> MSLFK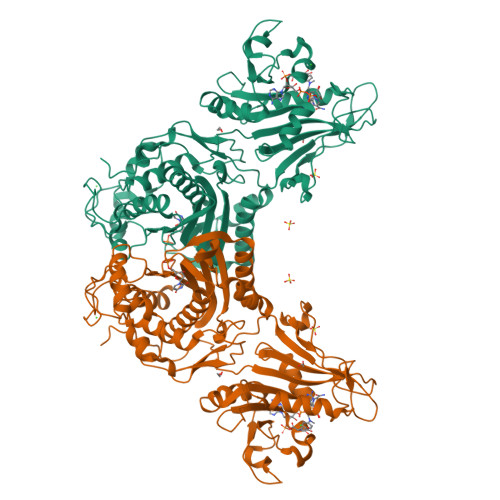IRMPETVAEGTRLALRAFSLVVAVDERGGIGDGRSIPWNVPEDMKFFRDVTTKLRGKNVKPSPAKRNAVVMGRKTWDSIPPKFRPLPGRLNVVLSSTLTTQHLLDGLPDEEKRNLHADSIVAVNGGLEQALQLLASPNYTPSIETVYCIGGGSVYAEALRPPCVHLLQAIYRTTIRASESSCSVFFRVPESGTEAAAGIEWQRETISEELTSANGNETKYYFEKLIPRNREEEQYLSLVDRIIREGNVKHDRTGVGTLSIFGAQMRFSLRNNRLPLLTTKRVFWRGVCEELLWFLRGETYAKKLSDKGVHIWDDNGSRAFLDSRGLTEYEEMDLGPVYGFQWRHFGAAYTHHDANYDGQGVDQIKAIVETLKTNPDDRRMLFTAWNPSALPRMALPPCHLLAQFYVSNGELSCMLYQRSCDMGLGVPFNIASYALLTILIAKATGLRPGELVHTLGDAHVYSNHVEPCNEQLKRVPRAFPYLVFRREREFLEDYEEGDMEVIDYAPYPPISMKMAV> MIDIHCHILPAMDDGAGDSADSIEMARAAVRQGIRTIIATPHH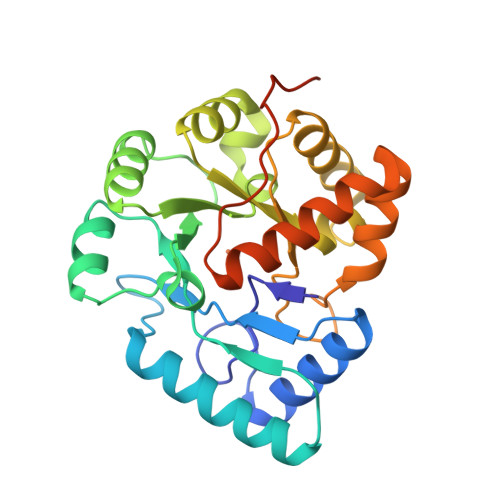NNGVYKNEPAAVREAADQLNKRLIKEDIPLHVLPGQEIRIYGEVEQDLAKRQLLSLNDTKYILIEFPFDHVPRYAEQLFYDLQLKGYIPVIAHPERNREIRENPSLLYHLVEKGAASQITSGSLAGIFGKQLKAFSLRLVEANLIHFVASDAHNVKTRNFHTQEALYVLEKEFGSELPYMLTENAELLLRNQTIFRQPPQPVKRRKLFGFFLEHHHHHH>[6x]MMSTTLFKDFTFEAAHRLPHVPEGHKCGRLHGHS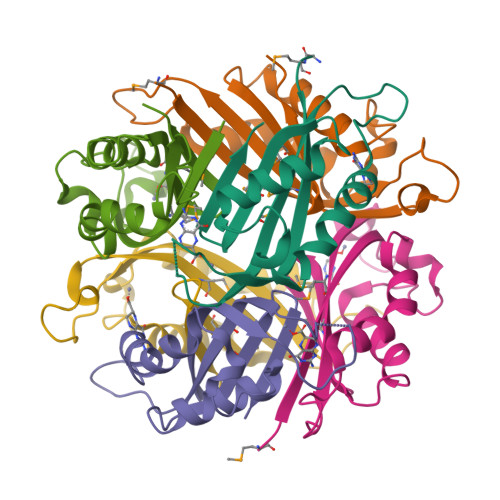FMVRLEITGEVDPHTGWIIDFAELKAAFKPTYERLDHHYLNDIPGLENPTSEVLAKWIWDQVKPVVPLLSAVMVKETCTAGCIYRGE>MDSDTDTDSGPVVATTKLV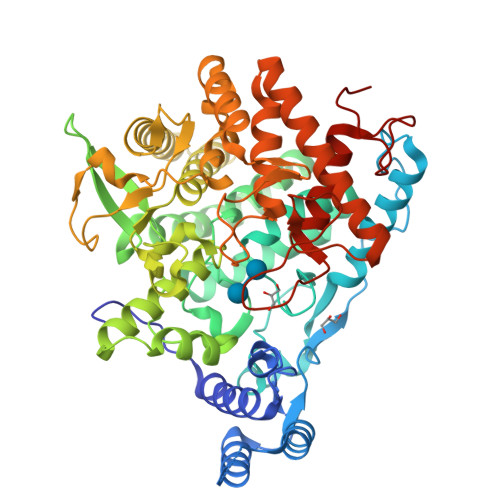TFLQRVQHTALRSYPKKQTPDPKSYIDLSLKRPYSLSTIESAFDDLTSESHDQPVPVETLEKFVKEYFDGAGEDLLHHEPVDFVSDPSGFLSNVENEEVREWAREVHGLWRNLSCRVSDSVRESADRHTLLPLPEPVIIPGSRFREVYYWDSYWVIKGLMTSQMFTTAKGLVTNLMSLVETYGYALNGARAYYTNRSQPPLLSSMVYEIYNVTKDEELVRKAIPLLLKEYEFWNSGKHKVVIRDANGYDHVLSRYYAMWNKPRPESSVFDEESASGFSTMLEKQRFHRDIATAAESGCAFSTRWMRDPPNFTTMATTSVVPVDLNVFLLKMELDIAFMMKVSGDQNGSDRFVKASKAREKAFQTVFWNEKAGQWLDYWLSSSGEESETWKAENQNTNVFASNFAPIWINSINSDENLVKKVVTALKNSGLIAPAGILTSLTNSGQQWDSPNGWAPQQEMIVTGLGRSSVKEAKEMAEDIARRWIKSNYLVYKKSGTIHEKLKVTELGEYGGGGEYMPQTGFGWSNGVILAFLEEYGWPSHLSIEALEHHHHHH[2x]>MSEFSQTVPELVAWARKNDFSISLPVDRLSFLLAVATLNGERLDGEMSEGELVDAFRHVSDAFEQTSETIGVRANNAINDMVRQRLLNRFTSEQAEGNAIYRLTPLGIGITDYYIRQREFSTLRLSMQLSIVAG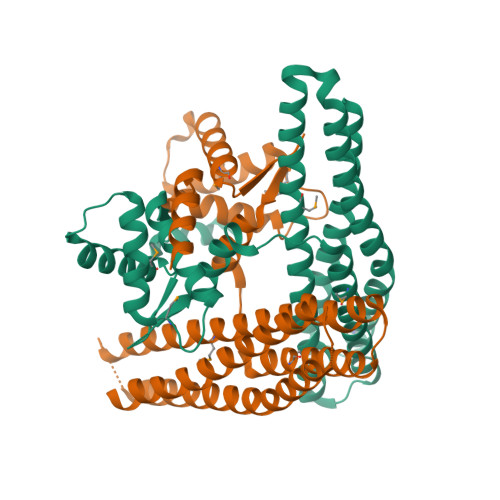ELKRAADAAEEGGDEFHWHRNVYAPLKYSVAEIFDSIDLTQRLMDEQQQQVKDDIAQLLNKDWRAAISSCELLLSETSGTLRELQDTLEAAGDKLQANLLRIQDATMTHDDLHFVDRLVFDLQSKLDRIISWGQQSIDLWIGYDRHVHKFIRT[2x]> MMGYIPYVIENTDRGERSYDIYSRLLKDRIVLLSGEINDSVASSIVAQLLFLEAEDPEKDIGLYINSPGGVITSGLSIYDTMNFIRPDVSTICIGQAA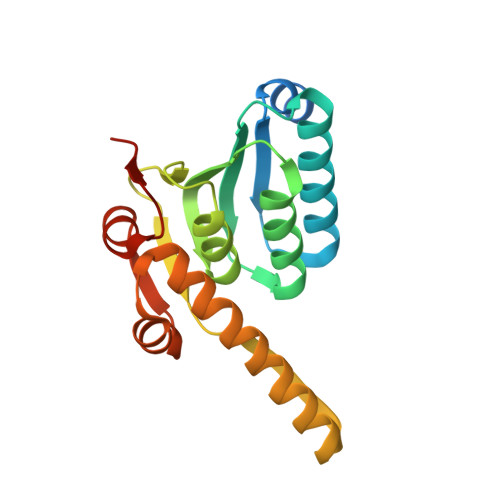AMGAFLLSCGAKGKRFSLPHSRIMIHQPLGGAQGQASDIEIISNEILRLKGLMNSILAQNSGQSLEQIAKDTDRDFYMSAKEAKEYGLIDKVLQKNVK> IESIIKTATDTVKSEINAELGVVPSLNAVETGATSNTEPEEAIQTRTVINQHGVSETLVENFLSRAALVSKRSFEYKDHTSSTAQTDKNFFKWTINTRSFVQLRRKLELFTYLRFDAEITILTTVAVNGSNNNTYVGLPDLTLQAMFVPTGALTPEKQDSFHWQSGSNASVFFKISDPPARMTIPFMCINSAYSVFYDGFAGFEKTGLYGINPADTIGNLCVRIVNEHQPVGFTVTVRVYMKPKHIKAWAPRPPRTLPYMSIANANYKGKERAPNALNAIIGNRDSVKTMPHNIV;> SPSAEACGYSDRVLQLKLGNSAIVTQEAANYCCAYGEWPNYLPDHEAVAIDKPTQPETATDRFYTLRSVKWEATSTGWWWKLPDALNNIGMFGQNVQHHYLYRSGFLIHVQCNATKFHQGALLVVAIPEHQRGAHNTTTSPGFDDIMKGEAGGTFNHPYVLDDGTSLACATIFPHQWINLRTNNSATIVLPWMNAAPMDFPLRHNQWTLAIIPVVPLGTRTMSSMVPITVSIAPMCCEFNGLRHAITQ;> GVPTYLLPGSGQFLTTDDHSSAPVLPCFNPTPEMHIPGQVRNMLEVVQVESMMEINNTESAVGMERLKVDISALTDVDQLLFNIPLDIQLDGPLRNTLVGNISRYYTHWSGSLEMTFMFCGSFMATGKLILCYTPPGGSCPTTRETAMLGTHIVWDFGLQSSITLIIPWISGSHYRMFNNDAKSTNANVGYVTCFMQTNLIVPSESSDTCSLIGFIAAKDDFSLRLMRDSPDIGQIDHLHGAEAAYQ;> MGAQVTRQQTGTHENANVATNGSHITYNQINFYKDSYAASASKQ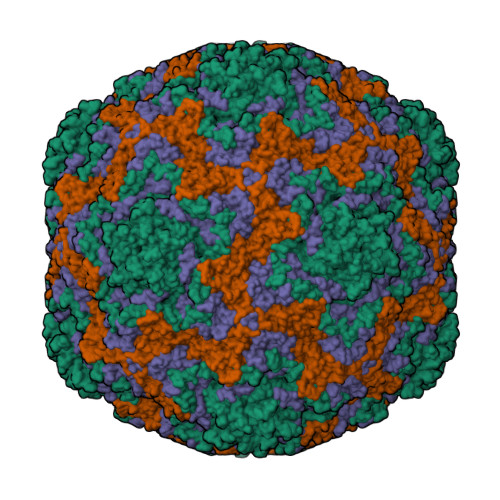DFSQDPSKFTEPVVEGLKAGAPVLK>[6x]MVSRYVPD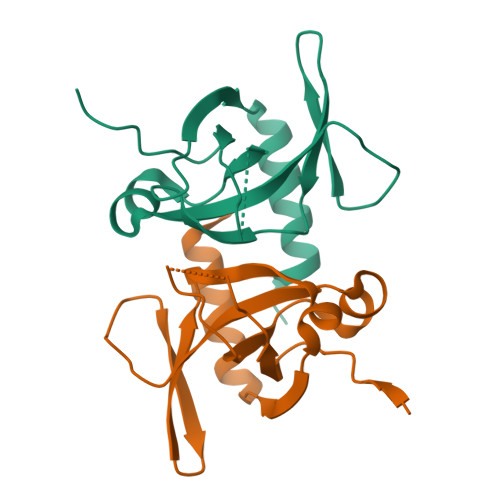MGDLIWVDFDPTKGSEQAGHRPAVVLSPFMYNNKTGMCLCVPCTTQSKGYPFEVVLSGQERDGVALADQVKSIAWRARGATKKGTVAPEELQLIKAKINVLIGHHHHHH>MYGWWGRILRVNLTTGEVKVQEYPEEVAKKFIGGRGLAAWILWNEARGVEPLSPENKLIFAAGPFNGLPTPSGGKLVVAAKSPLTGGYGDGNLGTMASVHLRRAGYDALVVEGKAKKPVYIYIEDDNVSILSAEGLWGKTTFETERELKEIHGKNVGVLTIGPAGENLVKYAVVISQEGRAAGRPGMGAVMGSKKLKAVVIRGTKEIPVADKEELKKLSQEAYNEILNSPGYPFWKRQGTMAAVEWCNTNYALPTRNFSDGYFEFARSIDGYTMEGMKVQQRGCPYCNMPCGNVVLDAEGQESELDYENVALLGSNLGIGKLNEVSVLNRIADEMGMDTISLGVSIAHVMEAVERGILKEGPTFGDFKGAKQLALDIAYRKGELGNLAAEGVKAMAEK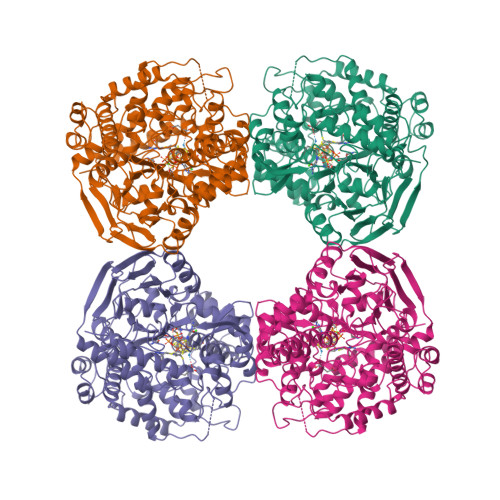LGTHDFAMHVKGLEVSGYNCYIYPAMALAYGTSAIGAHHKEAWVIAWEIGTAPIEGEKAEKVEYKISYDPIKAQKVVELQRLRGGLFEMLTACRLPWVEVGLSLDYYPKLLKAITGVTYTWDDLYKAADRVYSLIRAYWVREFNGKWDRKMDYPPKRWFTEGLKSGPHKGEHLDEKKYDELLSEYYRIRGWDERGIPKKETLKELDLDFVIPELEKVTNLE[4x]>ETGDKPLGETGTTGFQICKNALKLPVLEVLPGGGWDNLRNVDMGRVMDLTYTNCKTTEDGQYIIPDEVYTIPQKESNLEMNSEVLESWMNYQSTTSLSINTELALFSRVNGKFSTEFQRMKTLQVKDQAVTTRVQVRNRIYTVKTTPTSELSLGFTKALMDICDQLEKNQTKMATYLAELLILNYGTHVITSVDAGAALVQEDHVRSSFLLDNQNSQNTVTASAGIAFLNIVNFKVETDYISQTSLTKDYLSNRTNSRVQSFGGVPFYPGITLETWQKGITNHLVAIDRAGLPLHFFIKPDKLPGLPGPLVKKLSKTVETAVRHYYTFNTHPGCTNVDSPNFNFQANMDDDSCDAKVTNFTFGGVYQECTELSGDVLCQNLEQKNLLTGDFSCPPGYSPVHLLSQTHEEGYSRLECKKKCTLKIFCKTVCEDVFRVAKAEFRAYWCVAAGQVPDNSGLLFGGVFTDKTINPMTNAQSCPAGYIPLNLFESLKVCVSLDYELGFKFSVPFGGFFSCIMGNPLVNSDTAKDVRAPSLKKCPGGFSQHLAVISDGCQVSYCVKAGIFTGGSLLPVRLPPYTKPPLMSQVATNTVIVTNSETARSWIKDPQTNQWKLGEPLELRRAMTVIHGDSNGMSGGGTKTETSQVAPA[16x]

Perforin‐2 (PFN2, MPEG1) is a key pore‐forming protein in mammalian innate immunity restricting intracellular bacteria proliferation. It forms a membrane‐bound pre‐pore complex that converts to a pore‐forming structure upon acidification; but its mechanism of conformational transition has been debated. PFN2 belongs to the membrane attack complex‐perforin (MACPF) family and shares structural homology with bacterial cholesterol‐dependent cytolysins (CDCs; Gilbert et al, 2013). Distinct from MAC and perforin‐1, PFN2 is a type I transmembrane protein that is expected to be cleaved from its transmembrane anchor during bacterial restriction, releasing from the host membrane an ectodomain consisting of the MACPF and membrane‐binding P2 domain (McCormack & Podack, 2015).

Pore‐forming assemblies were prepared from pre‐pore oligomers pre‐assembled at pH 5.5, in which condition the bulk of the oligomers are complete full rings (Ni et al, 2020), and subsequently by lowering the pH to 3.6–4.0 in the presence of 0.056% Cymal‐6 (Ni et al, 2020). The isolated converted pores exist in two major conformations, a flat ring conformation (68.5%) and a twisted conformation (15.5%; Figs 3 and EV2), both structures comprising 16 mPFN2 subunits. The flat ring pore structure was resolved at an overall resolution ~ 3.0 Å with C2 symmetry, and with local resolutions ranging from 2.7 to 4.7 Å (Fig EV3). The ring pore follows C16 symmetry in the top of the MACPF domain, but its symmetry is gradually broken towards the bottom of the β‐barrel (Fig EV4A). It has an inner diameter of 75 Å at the top of the MACPF domain but a minimum and maximum diameter of 94 Å and 102 Å at the bottom, respectively. 3D variability analysis reveals that the top of the MACPF domain remains largely rigid in organization, presumably due to its large inter‐subunit buried surface area, while the bottom of the β‐barrel varies between circular and elliptical forms (Fig EV4A and Movie EV1). Compared with pre‐pore assemblies, several regions became unresolved, including the epidermal growth factor (EGF)‐like domain bridging the MACPF and P2 domains, and two β‐strands and an α‐helix in the very end of the CTT (residues S600 – I642, yellow in the pre‐pore). A loop between the P2 domain and CTT, which lies along the MACPF domain in pre‐pore oligomers, shifts to interact with its neighboring subunit (residues T581‐L590, red arrow). In addition, the P2 domain rotates ~ 90° around its pseudo‐3‐fold symmetry axis, and its β‐hairpin makes new contacts with the exterior of the β‐barrel now presented by the MACPF domain. The β‐barrel is further stabilized by a molecule of the detergent Cymal‐6, aligned with a strand from the P2 β‐hairpin and whose aliphatic region is packed with a series of hydrophobic residues from the back of the TMH barrel in the MACPF domain.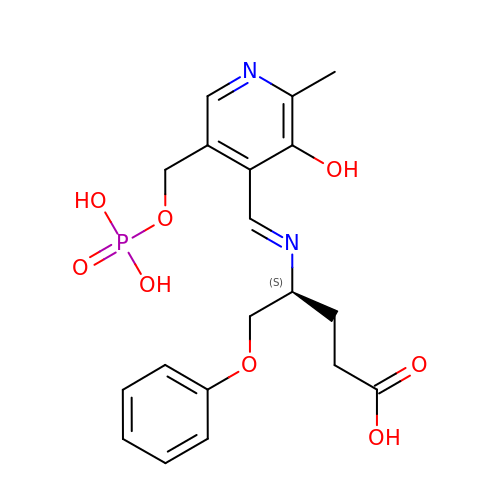(4S)-4-[(E)-({3-hydroxy-2-methyl-5-[(phosphonooxy)methyl]pyridin-4-yl}methylidene)amino]-5-phenoxypentanoic acid | C19 H23 N2 O8 P | HMMHDPPNPMIPCH-LKKXKRCMSA-N(2R)-4-AMINO-N-((1R,2S,3R,4R,5S)-5-AMINO-4-[(2-AMINO-2-DEOXY-ALPHA-D-GLUCOPYRANOSYL)OXY]-2-{2-[(3-AMINOPROPYL)AMINO]ETHOXY}-3-HYDROXYCYCLOHEXYL)-2-HYDROXYBUTANAMIDE 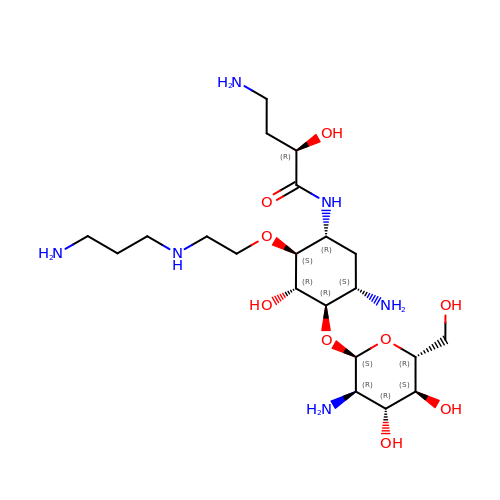| C21 H44 N6 O9 | MJKNCJCIMZKDAF-BORACOTDSA-N>MRNEMHLQFSARSENESFARVTVAAFVAQLDPTMDELTEIKTVVSEAVTNAIIHGYNNDPNGIVSISVIIEDGVVHLTVRDEGVGIPDIEEARQ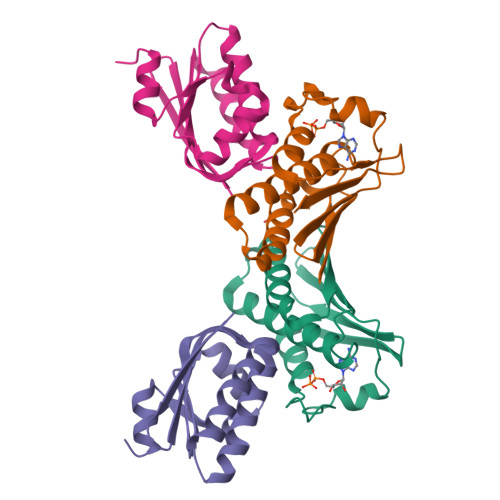PLFTTKPELERSGMGFTIMENFMDEVIVESEVNKGTTVYLKKHGIHHHHHH[2x];>[2x]MSLAIDLEVKQDVLIVRLSGELDHHTAEELREQVTDVLENRAIRHIVLNLGQLTFMDSSGLGVILGRYKQIKNVGGQMVVCAVSPAVKRLFDMSGLFKIIRVEADEQFALQALGVA> MNIKKFAKQATVLTFTTALLAGGATQAFAKETNQKPYKETYGISHITRHDMLQIPEQQKNEKYQVPEFDSS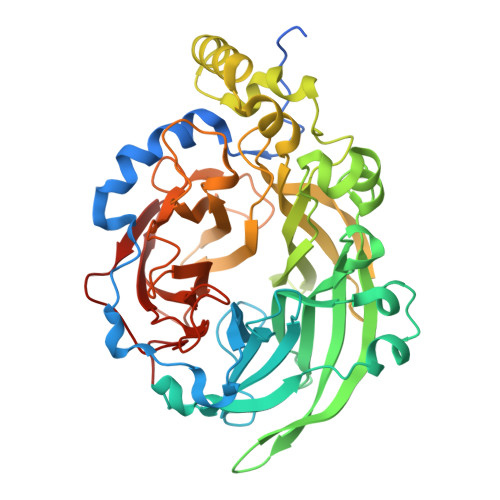TIKNISSAKGLDVWDSWPLQNADGTVANYHGYHIVFALAGDPKNADDTSIYMFYQKVGETSIDSWKNAGRVFKDSDKFDANDSILKDQTQEWSGSATFTSDGKIRLFYTDFSGKHYGKQTLTTAQVNVSASDSSLNINGVEDYKSIFDGDGKTYQNVQQFIDEGNYSSGDNHTLRDPHYVEDKGHKYLVFEANTGTEDGYQGEESLFNKAYYGKSTSFFRQESQKLLQSDKKRTAELANGALGMIELNDDYTLKKVMKPLIASNTVTDEIARANVFKMNGKWYLFTDSRGSKMTIDGITSNDIYMLGYVSNSLTGPYKPLNKTGLVLKMDLDPNDVTFTYSHFAVPQAKGNNVVITSYMTNRGFYADKQSTFAPSFLLNIKGKKTSVVKDSILEQGQLTVNK>[2x]LVPAGSHMMKTLSLQSRAKTTALKQPKEIFAFARDIDGEFVYDQKIVKDENVSYYYLPDSKIDG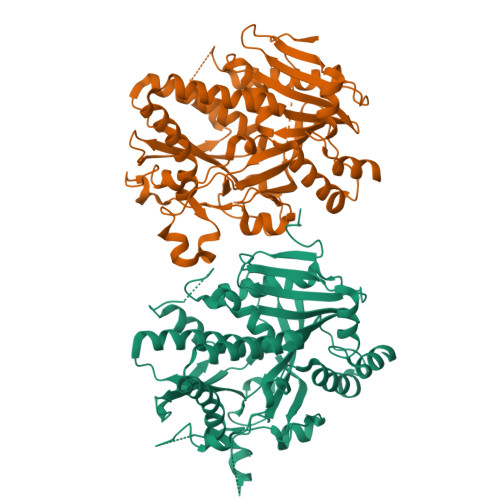SIDLQAGYAKFKKIPEEKNMSDMKCLLTALTKYEQEHNNGEKVNVDIITYRGLMTKLLALPYNLNDPVDLNVLAYDGQLFINSDEEIELARRKEEDEHKQQSMTPEKYDHMKRCEFSGYKFEAIATLPKPWADCSRQQIDKRGKKMVNNYEQYISVIKTGIGEAKMLLAGEVDCVWDYIPEDGKDVLSHYMELKTTRILESNGQVVNFEKKLFKTWAQCFLMGIRKVVYGFRDDSFFLRDVELYKTEEIPLLIKNNALTENKSGGKINCTTALKWYGAVIEWLLQEIPRDDTSKAYRVSFDPSTRTFTLRELMGNENSRLRNGEMLTSEFKQWRESIQK(2E)-2-methyl-4-(9H-purin-6-ylamino)but-2-en-1-ol | C10 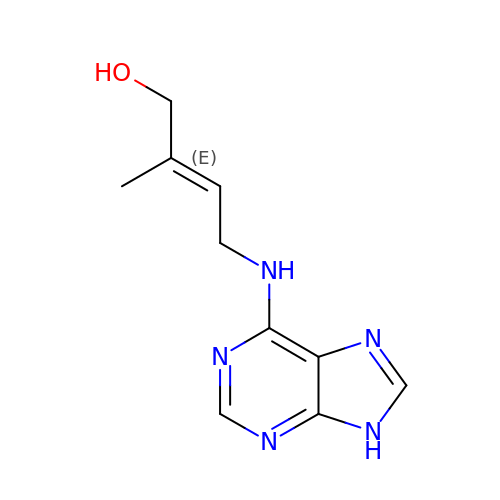H13 N5 O | UZKQTCBAMSWPJD-FARCUNLSSA-N>[2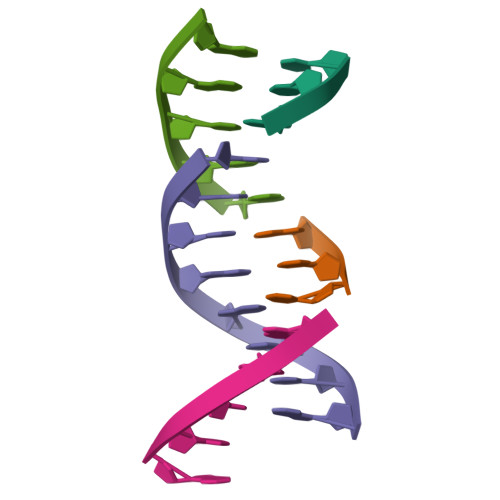x]CCG;> ATCGGCCG;>[2x]ATCGG> MTGPTRAL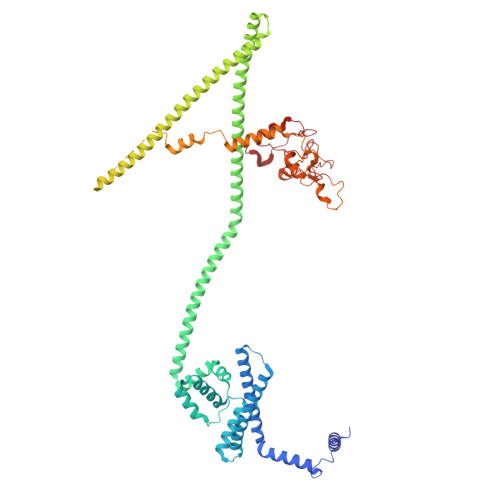FLSSGINLGRLRLAEQFSSMNGWQSKEDPAFDAYVKERRRKENYEAFDQRVERGYAAAAKLHKAEIQNAVKRRLKSSGAKFTAETLREMSSAVTERLAWLRDVWAQIDADYRSGDSARQETAAQEISAALRGEPNDYMRWVYETKRELRFAGPVGRRAIQEELQAAELPEVLDEEVNRYHDLKLNMMEIEREVKAKYGVAGQQHWAELQAAKDEEYIQKLDEAAEVYKQLLDQSARLDESRRSELQRSYVERVHQAQVRFKAAMELEGQREQLIEAHQAMKEERMRTEREKRRQLLREAAELRAQGKKSADVLTALKERQLDANAKRQAEYELKECEDILKRKSEMLDMIAHFKHDVEEREGREMLQRQKSDERQVNVFGFYEEVGVEDGLSISSEGTTSQGGSSGLGTVSTSTSCAKSADSNSSAQPSQKLRKEELWKVINADTYEDPFRTVHQARLDAVKTYDPAYARTFPLNLVLGRKYSRQGAGEMAAGNETDKQILQKGNNILYSFQWGLNNGTVHDLDADGGTDYFMDGAFHVRDKETGDIDWRYEKKRGGPVFRGPKFYRLGAQREAADPGERAMDPTPYTSTPREHKWRSS The C-type mannose receptor and its homolog Endo180 (or uPARAP, for urokinase plasminogen activator receptor-associated protein) mediate the endocytic uptake of collagen by macrophages and fibroblasts. The large extracellular region of each of these receptors consists of an N-terminal ricin B-like domain, followed by a fibronectin type II (FN2) domain and eight (MR, Endo180, PLA2R) or ten (DEC-205) C-type lectin (CTL) domains. Here, we present the crystal and solution structures of domains 1–4 (D1-4) of Endo180 and a mutational analysis of collagen binding. The Endo180 D1-4 region adopts an L-shaped structure with a short arm (∼60 Å length) consisting of the ricin-like and FN2 domains, and a longer arm (∼80 Å length) consisting of the two CTL domains.

We obtained two crystal forms of the natively glycosylated D1-4 region, one of which diffracted to 2.5 Å resolution and allowed the structure to be determined. The overall structure of Endo180 D1-4 is the same in both crystal forms (the root-mean-square deviations [rmsd] between the four crystallographically independent copies range from 1.2 to 1.4 Å) and only the high-resolution structure is described in the following.

>[2x]APLADAALPEPNVFLIFSHGLQGCLEAQGGQVRVTPACNTSLPAQRWKWVSRNRLFNLGTMQCLGTGWPGTNTTASLGMYECDREALNLRWHCRTLGDQLSLLLGARTSNISKPGTLERGDQTRSGQWRIYGSEEDLCALPYHEVYTIQGNSHGKPCTIPFKYDNQWFHGCTSTGREDGHLWCATTQDYGKDERWGFCPIKSNDCETFWDKDQLTDSCYQFNFQSTLSWREAWASCEQQGADLLSITEIHEQTYINGLLTGYSSTLWIGLNDLDTSGGWQWSDNSPLKYLNWESDQPDNPSEENCGVIRTESSGGWQNRDCSIALPYVCKKKPNATAEPTPPDRWANVKVECEPSWQPFQGHCYRLQAEKRSWQESKKACLRGGGDLVSIHSMAELEFITKQIKQEVEELWIGLNDLKLQMNFEWSDGSLVSFTHWHPFEPNNFRDSLEDCVTIWGPEGRWNDSPCNQSLPSICKKAGQLSGAAAHHHHHH>[8x]MASWSHPQFEKIEGRRDRGPEFELGTENLFFEGETIAIVGGTLIDGNGGVPVPETTVFIEDGRITKVGSTDQIEVHPNIRQIDAQGKWILPGLVNGNVHLLDGIMMMGRGGIEYLARFEGNYYKVIEEAAQIALRGGVTTVFDTWNALEPVTIARDRIASGAAEGARIFFAGTLIGMGGPFTGDFMRPSMQARTVMSRTFADRMDAMFEVGMGRHLSTLPPAE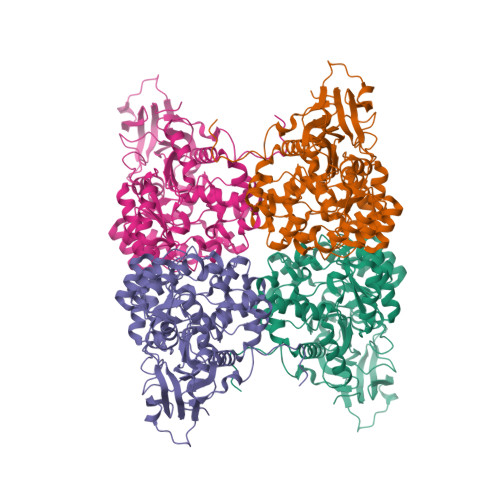VRPLIREYLERGVDFCKIAVTDHLVGLLGFRAPYFTFSERVLDVLVDEVRRAGVPLLTHTTSLEGLNTAIERDADLMIHATMTGQAPIPEETIEKLLEKQLWSEVQPTTIAQQAWMDSVDHPFADFSGRVHHENDVRMIKAGVPLVLGTDAGCTDPDILEDMSQGELHERPWTLGEDHFVWMQAMVEKGMDPMAAILAGTANPAKAYRKFDELGSIDVGKLGDVVVLDQDPLADITNMRTLSHVVKEGREIDFHGLPLSPLVTAYPRTANVLD> AAESGVSRPVPQLKRTTMRILIGLLVQNPELATLVPPLENLDENKLPGLGLFRELVNTCLSQPGLTTGQLLEHYRGTNNAATLEKLSMWDDIA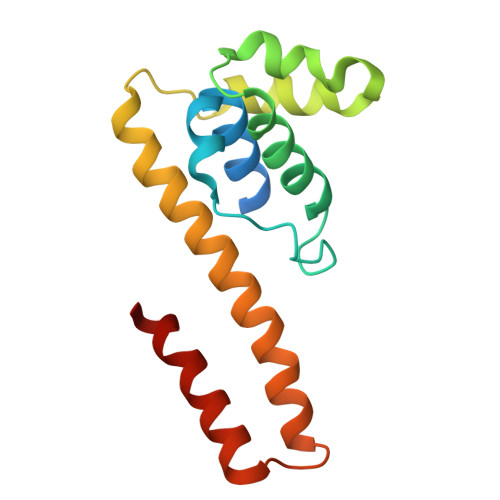DKNIAEQTFTDSLNHMFDSLLELRQEELIARERTHGLSNEECLELWTLNQELAKK>HHHHHHMQHLVLIGFMGSGKSSLAQELGLALKLEVLDTDMIISERVGLSVREIFEELGEDNFRMFEKNLIDELKTLKTPHVISTGGGIVMHENLKGLGTTFYLKMDFETLIKRLNQKEREKRPLLNNLTQAKELFEKRQALYEKNASFIIDARGGLNNSLKQVLQFIA[2x]

SK catalyzes the specific phosphorylation of the 3-hydroxyl group of shikimic acid, using ATP as a co-substrate. The shikimate pathway is comprised of seven enzymatic components that convert erythrose 4-phosphate and phosphoenolpyruvate into chorismate, for subsequent synthesis of aromatic compounds. SKs belong to a class of P-loop kinases that share a homologous α-β-α fold. Overall, these structures have a characteristic α-β-α fold that consists of the CORE domain (residues 1–31, 61–108, and 124–162), the SB domain (residues 32–60), and the LID region (residues 109–123) in the monomer.

Here, we additionally determined structures of a dimeric HpSK·SO4 (R = 22.7%, Rfree = 26.0%), HpSK• S3P•ADP (R = 23.1%, Rfree = 27.7%), and R57A (R = 24.6%, Rfree = 27.3%). For the dimeric HpSK·SO4 structure, the LID region points upward, and a number of residues cannot be built into this region (residues 108–118 in subunit A, and 111–117 in subunit B), implying a disordered region. The LID region is most flexible and flips over the binding pocket, in an open or closed state. In the open form, HpSK (flexible LID) presents a wide-opening pocket, allowing entry of promising substrates.>MRGSPHHHHHHGSAKNVVLDHDGNLDDFVAMVLLASNTEKVRLIGALCTDADCFVENGFNVTGKIMCLMHNNMNLPLFPIGKSAATAVNPFPKEWRCLAKNMDDMPILNIPENVELWDKIKAENEKYEGQQLLADLVMNSEEKVTICVTGPLSNVAWCIDKYGEKFTSKVEECVIMGGAVDVRGNVFLPSTDGTAEWNIYWDPASAKTVFGCPGLRRIMFSLDSTNTVPVRSPYVQRFGEQTNFLLSIL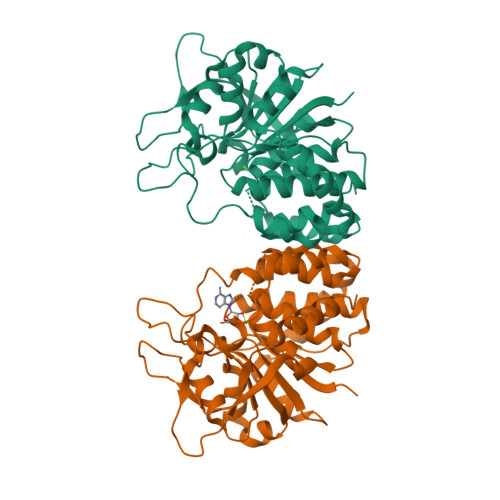VGTMWAMCTHCELLRDGDGYYAADALTAAYVVDQKVANVDPVPIDVVVDKQPNEGATVRTDAENYPLTFVARNPEAEFFLDMLLRSARAC[2x]>[6x]MERLRQIASQATAASAAPARPAHPLDPLSTAEIKAATNTVKSYFAGKKISFNTVTLREPARKAYIQWKEQGGPLPPRLAYYVILEAGKPGVKEGLVDLASLSVIETRALETVQPILTVEDLCSTEEVIRNDPAVIEQCVLSGIPANEMHKVYCDPWTIGYDERWGTGKRLQQALVYYRSDEDDSQYSHPLDFCPIVDTEEKKVIFIDIPNRRRKVSKHKHANFYPKHMIEKVGAMRPEAPPINVTQPEGVSFKMTGNVMEWSNFKFHIGFNYREGIVLSDVSYNDHGNVRPIFHRISLSEMIVPYGSPEFPHQRKHALDIGEYGAGYMTNPLSLGCDCKGVIHYLDAHFSDRAGDPITVKNAVCIHEEDDGLLFKHSDFRDNFATSLVTRATKLVVSQIFTAANYEYCLYWVFMQDGAIRLDIRLTGILNTYILGDDEEAGPWGTRVYPNVNAHNHQHLFSLRIDPRIDGDGNSAAACDAKSSP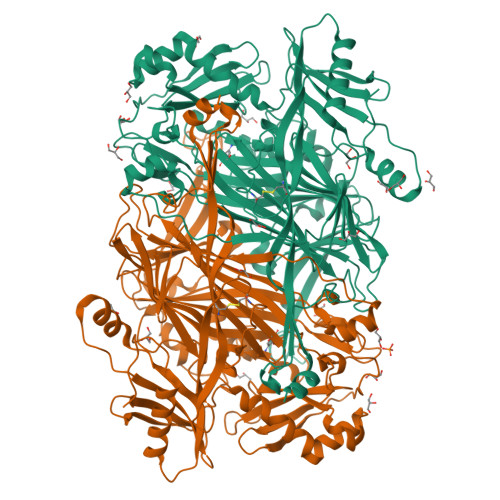YPLGSPENMYGNAFYSEKTTFKTVKDSLTNYESATGRSWDIFNPNKVNPYSGKPPSYKLVSTQCPPLLAKEGSLVAKRAPWASHSVNVVPYKDNRLYPSGDHVPQWSGDGVRGMREWIGDGSENIDNTDILFFHTFGITHFPAPEDFPLMPAEPITLMLRPRHFFTENPGLDIQPSYAMTTSEAKRAVHKETKDKTSRLAFEGSCCGK> GSMLDFSKDFLFGVATASYQVEGAYNEDGRTMSIWDTFSRQDGKVYKSHNGDVACDHYHLYKDDVKMMKDLGIEAYRFSIAWPRIFPAKGQYNPKGMDFYKRLTDELLKNDIKPFATIYHWDLPQWADDLGGWLNREIVEWYGEYAEKLFSELGGYIKNWITLNEPWCSSFLSYFIGEHAPGHKDLGEALLVSHNLLLSHGKAVEIFRGLNLDDSKIGITLNLNEVFPASDSDDDKVAAQIADGFQNRWFLDPLFKGKYPQDMVEYFGKYAKVDFINDEDLKLIS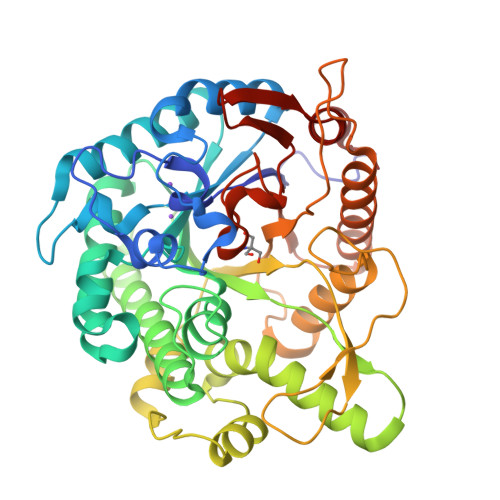QKLDFLGVNYYTRAVVQKGNDGLLDAVQIDPGNERTEMGWEIYPESLYNILMRLKREYTYDMPLYITENGAAFNDVVEDDGRVHDEKRVEFLKQHFKEAKRFLNDGGNLKGYFVWSLMDNFEWAHGYSKRFGIVYVDYETEKRILKDSALWYKDLISTRTI>[2x]MDHLPIFCQLRDRDCLIVGGGDVAERKARLLLEAGARLTVNALTFIPQFTVWANEGMLTLVEGPFDETLLDSCWLAIAATDDDTVNQRVSDAAESRRIFCNVVDAPKAASFIMPSIIDRSPLMVAVSSGG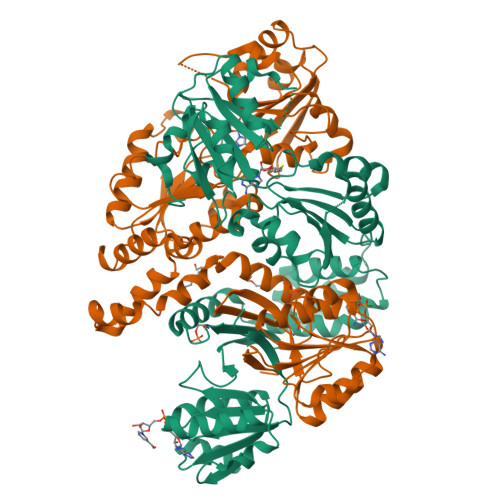TSPVLARLLREKLESLLPQHLGQVARYAGQLRARVKKQFATMGERRRFWEKFFVNDRLAQSLANADEKAVNATTERLFSEPLDHRGEVVLVGAGPGDAGLLTLKGLQQIQQADIVVYDRLVSDDIMNLVRRDADRVFVGKRAGYHCVPQEEINQILLREAQKGKRVVRLKGGDPFIFGRGGEELETLCHAGIPFSVVPGITAASGCSAYSGIPLTHRDYAQSVRLVTGHLKTGGELDWENLAAEKQTLVFYMGLNQAATIQEKLIAFGMQADMPVALVENGTSVKQRVVHGVLTQLGELAQQVESPALIIVGRVVALRDKLNWFSNH>MITFIGHVSKDVNVVDGKREIAYGGGVVMGAITSSLLGVKTKVITKCTREDVSKFSFLRDNGVEVVFLKSPRTTSIENRYGSDPDTRESFLISAADPFTESDLAFIEGEAVHINPLWYGEFPEDLIPVLRRKVMFLSADAQGFVRVPENEKLVYRDWEMKEKYLKYLDLFKVDSREAETLTGTNDLRESCRIIRSFGAKIILATHASGVIVFDG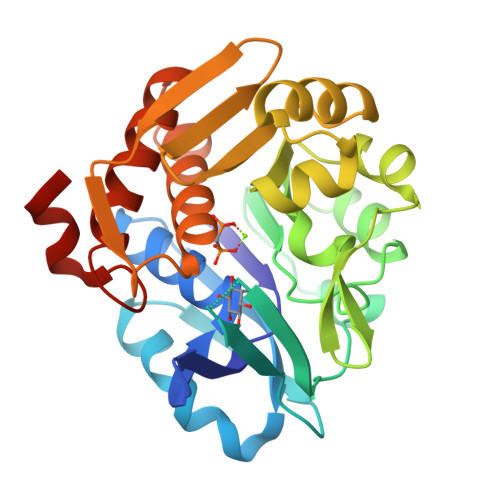NFYEASFRSWSLEGRTGRGDTCTAAFLVGFVFKKMSIEKATKFAAAVTSVKMRHPGPLRREDLEAISGDQYF[2x]PB1 domains are protein interaction modules with critical roles in the assembly of protein complexes involved in autophagy, signaling, cell division, and redox processes, as well as the auxin-response pathway in plants. PB1 domains form homotypic interactions via conserved electrostatic motifs molded by basic or acidic surface patches on opposite faces of their ubiquitin-like β-grasp fold. While type A and type B PB1 domains can form heterodimeric protein complexes, type AB members can mediate interactions with either PB1 domain type or engage in homotypic interactions to form homo-oligomers or hetero-oligomers. Our cryo-EM structures of filamentous p62 and AtNBR1–PB1 assemblies revealed that the presence of a tandem arginine sequence in the basic motif of type AB interfaces is required to stabilize a polymeric assembly.

In the absence of prior structural information, we traced the AtNBR1–PB1 de novo. This de novo-built model is in close agreement with the 1.6-Å crystal structure of a polymerization-deficient AtNBR1–PB1 mutant, which we solved in parallel. To validate our structural interpretation, we performed pull-down experiments using MBP-tagged wild-type AtNBR1–PB1 as a prey and a series of AtNBR1–PB1 interface mutants as bait. All interface mutants decrease binding significantly compared with the wild type, and binding is completely abrogated in mutants lacking the double arginine finger, in agreement with observations in cellular assays.

> MESTANALVVKVSYGGVLRRFRVPVKANGQLDLEMAGLKEKIAALFNLSADAELSLTYSAADGAVVALVDDNDLFDVTNQRLKFLKINVNAGVS>MTSQPVPHPSARHSHAHPHVHSQESLQKLVNRLSRIEGHIRGVKTMVQENRPCPEVLIQVAAVRGALDRVARLILDDHMNECITRAAAEGNIEQELAELKEALDR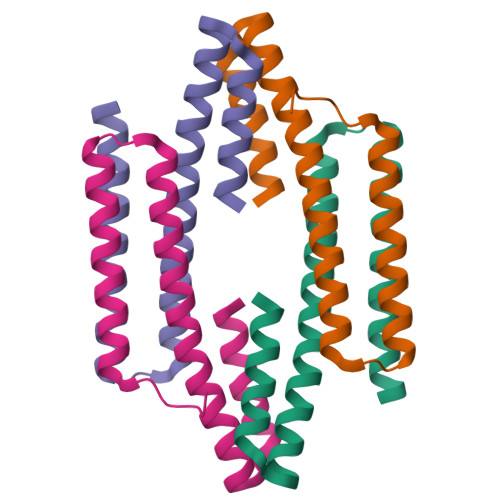FL[2x]>[2x]MPDVDWNMLRGNATQAAAGAYVPYSRFAVGAAALVDDGRVVTGCNVDNVSYGLTLCAECAVVCALHSTGGGRLLALACVDGHGSVLMPCGRCRQVLLEHGGSELLIDHPV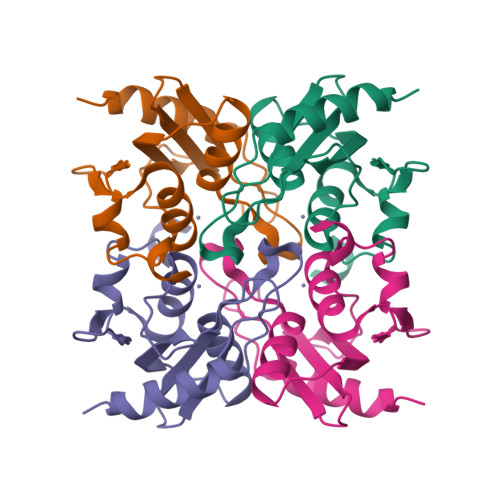RPRRLGDLLPDAFGLDDLPRERR>[2x]MGRGSHHHHHHGMAMNIKELSLHELCEELKTPAWNVPLTFVGDVGGTSARMGFVREGKNDSVHACVTRYSMKRKDITELIEFFNEIIELMPASVIKRVKAGVINVPGPVTGGAVGGPFNNLKGIARLSDYPKALFPPGRSAILNDLEAGGFGVLAVSDAHVFSEYFGVMWEGTQWRTCEQEPAGSVIGRGRCLVLAPGTGLGSSLIYYNPMNQQHIVVPLELGSQTIPMRKDIDY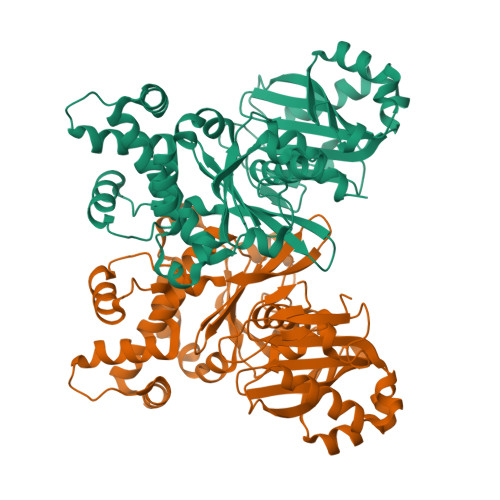IQTLHAELKLLPNYENMVSGAGLEFHYRQVVRGSRPPCSAGEIAKLASEGDANACKAMKKYHEYLMRVGSEASMALLPLTIVLVGDNIVNNAFFYRNPQNLKEMHREALNHEMERAGFQSRVTYLRQKKLLNLNLMGCYRCGLDLS> VETRTIVRFNR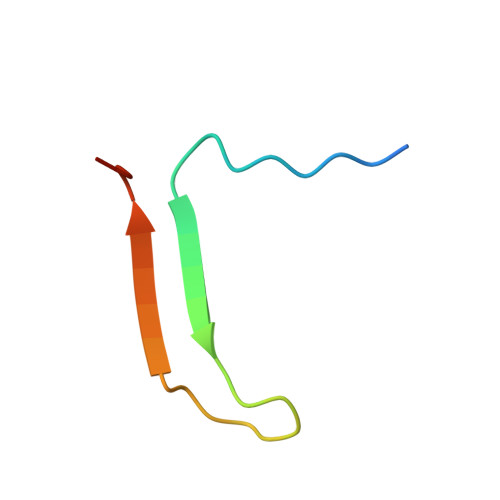PFLMIIVPTDTQNIFFMSKVTNPKQA3-[[4-imidazol-1-yl-6-[(3~{R})-3-oxidanylpyrrolidin-1-yl]-1,3,5-triazin-2-yl]amino]-4-methyl-~{N}-[3-(trifluoromethyl)phenyl]benzamide | 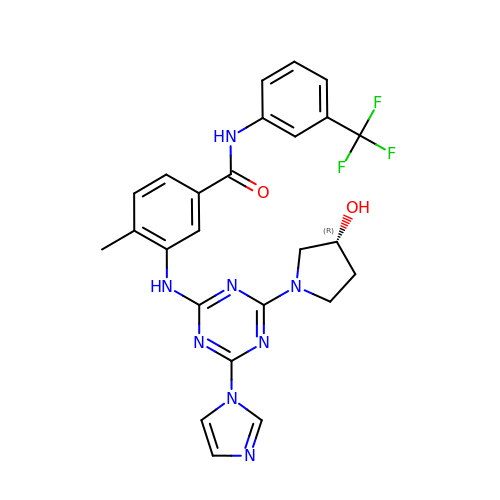C25 H23 F3 N8 O2 | IOGRLXUUAIVKHX-LJQANCHMSA-N2'-DEOXYADENOSINE 5'-TRIPHOSPHATE | 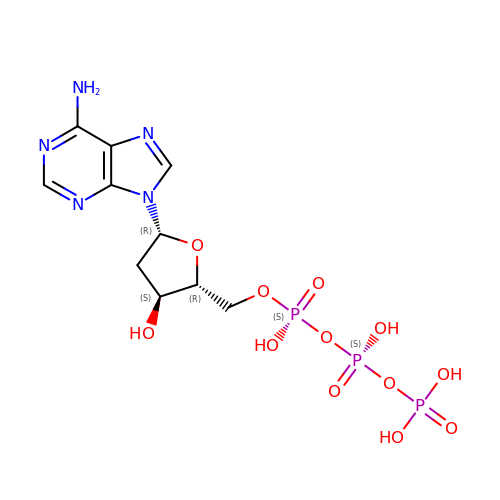C10 H16 N5 O12 P3 | SUYVUBYJARFZHO-RRKCRQDMSA-N> GPLGSSQIPAS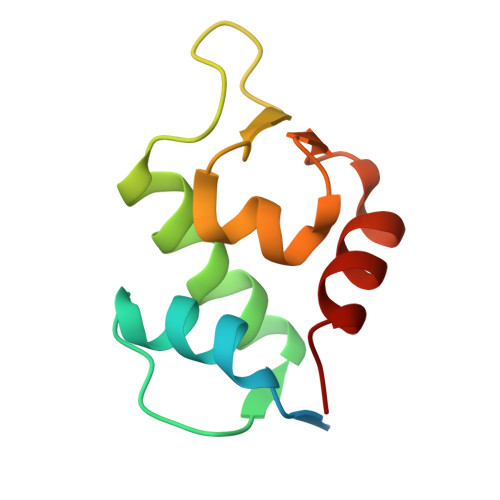EQETLVRPKPLLLKLLKSVGAQKDTYTMKEVLFYLGQYIMTKRLYDAAQQHIVYCSNDLLGDLFGVPSFSVKEHRKIYTMIYRNLV>MGHHHHHHHHHHHMAQGTLIRVTPEQPTHAVCVLGTLTQLDICSSAPEDCTSFSINASPGVVVDIAHGPPAKKKSTGSSTWPLDPGVEVTLTMKVASGSTGDQKVQISYYGPKTPPVKALLYLTGVEISLCADITRTGKVKPTRAVKDQRTWTWGPCGQGAILLVNCDRDNLESSAMDCEDDEVLDSEDLQDMSLMTLSTKTPKDFFTNHTLVLHVARSEMDKVRVFQATRGKLSSKCSVVLGPKWPSHYLMVPGGKHNMDFYVEALAFPDTDFPGLITLTISLLDTSNLELPEAVVFQDSVVFRVAPWIMTPNTQPPQEVYACSIFENEDFLKSVTTLAMKAKCKLTICPEEENMDDQWMQDEMEIGYIQAPHKTLPVVFDSPRNRGLKEFPIKRVMGPDFGYVTRGPQTGGISGLDSFGNLEVSPPVTVRGKEYPLGRILFGDSCYPSNDSRQMHQALQDFLSAQQVQAPVKLYSDWLSVGHVDEFLSFVPAPDRKGFRLLLASPRSCYKLFQEQQNEGHGEALLFEGIKKKKQQKIKNILSNKTLREHNSFVERCIDWNRELLKRELGLAESDIIDIPQLFKLKEFSKAEAFFPNMVNMLVLGKHLGIPKPFGPVINGRCC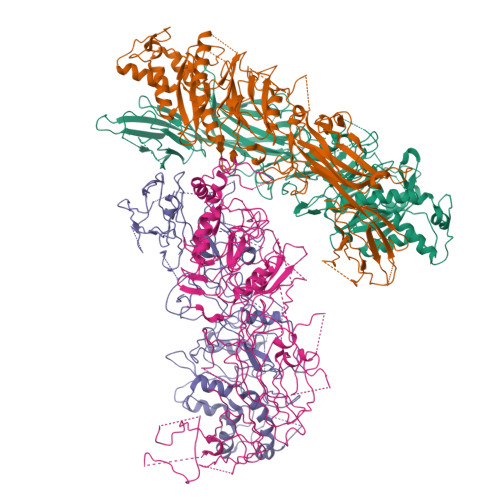LEEKVCSLLEPLGLQCTFINDFFTYHIRHGEVHCGTNVRRKPFSFKWWNMVP[4x]1,3-dihydroxypropan-2-yl (5Z,8Z,11Z,14Z)-icosa-5,8,11,14-tetraenoate | C23 H38 O4 | 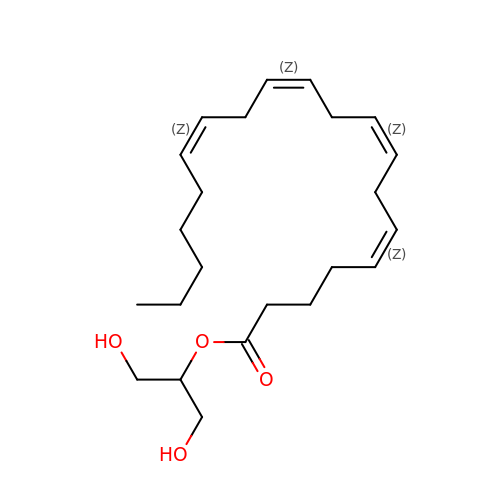RCRCTBLIHCHWDZ-DOFZRALJSA-N>HHHHHHSSGLVPRGSHMASQVVRIVGVGRTGIGKLHKSVDELAASALKCALVDANMKQCDLQALIAVPSLASPQFMQAHHIATVAGLFPTKGKFIVRTVDTGGAGPITALGMAVDLVRTRCAETVAVIAADAVLSMGSGAFAERSNASLRRSGLPEPCIPHGYDRYAQWYMSRYGLKREQLAMVPVLMSKMAERHPEAMCQKAYTLDEVLHSRCVAPVTNLLECARRADGAVALIVSGEAHYAEHFAQGKQEQRHLGGSKPIIASVAEASGPLFPPGSSDDIVPDIFSCRHAARDAFLSANLNVGDIHFF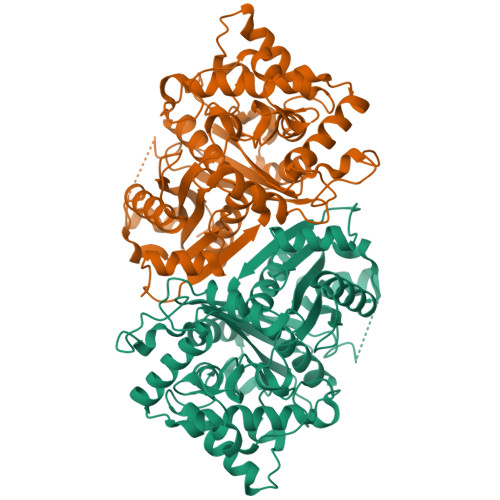GLYDCFPICLIQAVEAVGLCPEGKGGEFMETAYNEMLNNGGVLDPSKFPINTHGGLQCFGAPWEVPAMYNITEAIAQLSEEAGDRQLTPVPKRALVYGNGGIFSASSVAILISDL[2x]> MAGPRPVVLSGPSGAGKSTLLKKLFQEHSSIFGFSVSHTTRNPRPGEEDGKDYYFVTREMMQRDIAAGDFIEHAEFSGNLYGTSKEAVRAVQAMNRICVLDVDLQGVRSIKKTDLCPIYIFVQPPSLDVLEQRLRLRNTETEESLAKRLA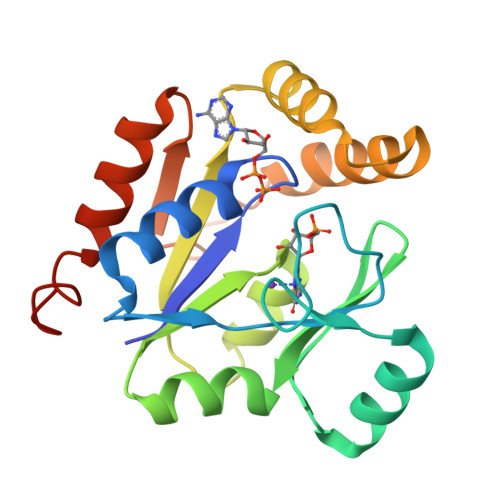AARTDMESSKEPGLFDLVIINDDLDKAYATLKQALSEEIKKAQGTGHA> SASYKPVFVTEITDDLHFYVQDVETGTQFEKLMENMRNDIASHPPVEGSYAPRRGEFCIAKFVDGEWYRARVEKVESPAKIHVFYID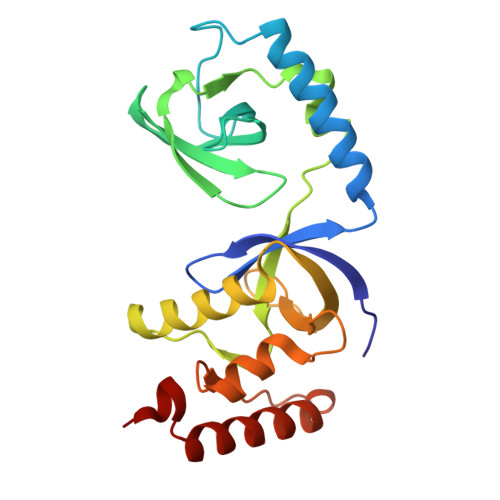YGNREVLPSTRLGTLSPAFSTRVLPAQATEYAFAFIQVPQDDDARTDAVDSVVRDIQNTQCLLNVEHLSAGCPHVTLQFADSKGDVGLGLVKEGLVMVEVRKEKQFQKVITEYLNAQESAKSARLNLWRY> MGMPVPGTLSVEIPPRYCPLPTARHPDETVLARRTADWIDGFDLELTPQQRARMRGNDCPGFYGRIMPHSPTDRLQLAVDWCTVMFHFDDVHCDEGPATGRAARFADLATRIVRVLEAPDARLEGPGDTMLAPVRDLALRARRWATPAQMRRCAEAHRAWFLAVAWELGHRAARSTPALNDY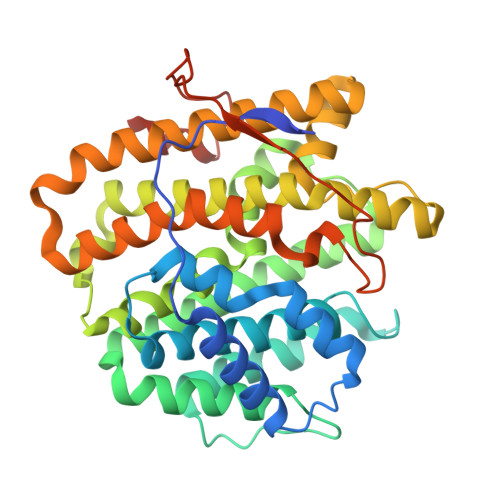AHMRQHTAAGAATLAWAEIVDGAEIPDRELSSPEVRALTELAFTTAAFDDDLFSYGKELWVARAEGTAPSGLGLVEILRRENRCGRPEALRAAVCLCNRLTHRFIALRERVLPDASAPLRAYLDHLCHLLPGNLEWGLTADRYRNPDGRTPGAVTTTASRDTDPPADTSPPAIPSIAWWWDPLGGRPATEHHHHHH> MSHQERLQSKSLHLSPQEQSASYQDRRQSWRRASMKETNRRKSLHPIHQGITELSRSISVDLAESKRLGCLLLSSFQFSIQKLEPFLRDTKGFSLESFRAKASSLSEELKHFAD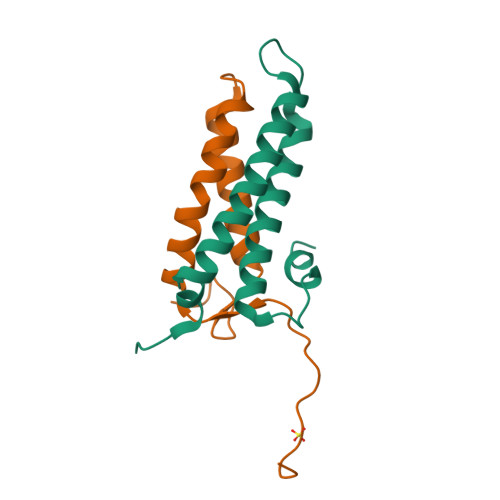GLETDGTLQKCFEDSNGKAS;> GPLGSSATPREDFRVRCTSKRAVTEMLQLCGRFVQKLGDALPEEIREPALRDAQWTFESAVQENISINGQAWQEAS>HMDTTFQAAIDTGKINGAVVCATDAQGHFVYNKATGERTLLSGEKQPQQLDDVLYLAAATKLITTIAALQCVEDGLLSLDGDLSSIAPELAAKYVLTGFTDDESPLDDPPARPITLKMLLTHSSGTSYHFLDPSIAKWRAQYANPENEKPRLVEEMFTYPLSFQPGTGWMYGPGLDWAGRVVERVTGGTLMEFMQKRIFDPLGITDSQFYPVTREDLRARLVDLNPSDPGALGSAVIGGGGEMNLRGRGAFGGHGLFLTGLDFVKILRSLLANDGMLLKPAAVDNMF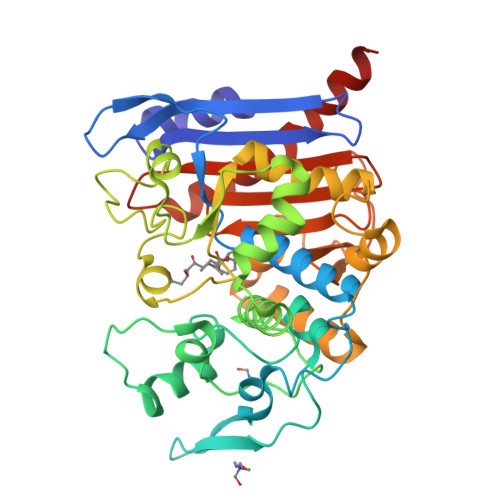QQHLGPEAAASHRAALASPLGPFFRVGTDPETKVGYGLGGLLTLEDVDGWYGERTLTWGGGLTLTWFIDRKNNLCGVGAIQAVLPVDGDLMADLKQTFRHDIYRKYSAWKGQQ[2x]>MHHHHHHSSGLVPRGSHMISKEYHIDEEVGFALPNPQENLPDFYNDWMFIAKHLPDLIESGQLRERVEKLNMLSIDHLTDHKSQRLARLVLGCITMAYVWGKGHGDVRKVLPRNIAVPYCQLSKKLELPPILVYADCVLANWKKKDPNKPLTYENMDVLFSFRDGDCSKGFFLVSLLVEIAAASAIKVIPTVFKAMQMQERDTLLKALLEIASCLEKALQVFHQIHDHVNPKAFFSVLRIYLSGWKGNPQLSDGLVYEGFWEDPKEFAGGSAGQSSVFQCFDVLLGIQQTAGGGHAAQFLQDMRRYMPPAHRNFLCSLESNPSVREFVLSKGDAGLREAYDACVKALVSLRSYHLQIVTKYILIPASQQPKENKTSEDPSKLEAKGTGG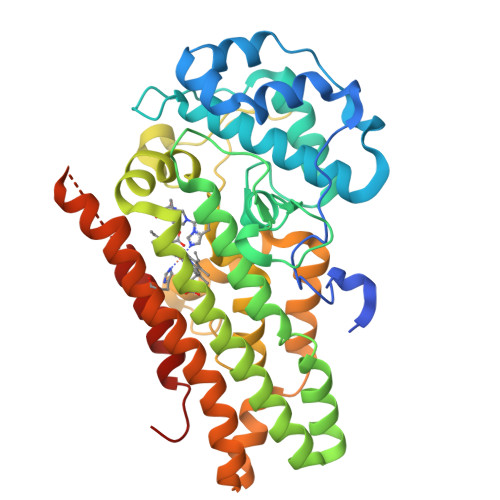TDLMNFLKTVRSTTEKSLLKEG[2x]> MADEIAKAQVARPGGDTIFGKIIRKEIPAKIIFEDDQALAFHDISP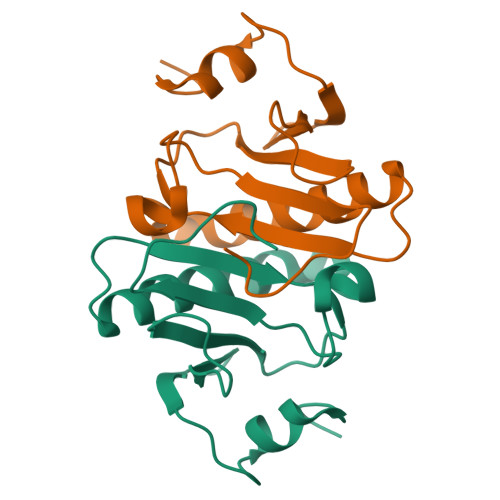QAPTHFLVIPKKHISQISAAEDADESLLGHLMIVGKKAAADLGLKKGYRMVVNEGSDGGQSVYHVHLHVLGGRQMNWPPG>[2x]GSHMSI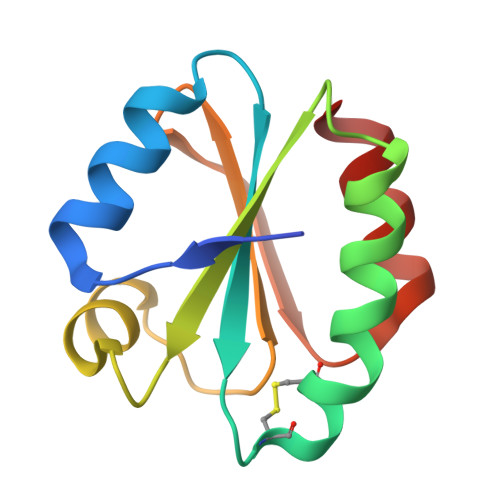HIKDSDDLKTRLAEAGDKLVVIDFMATWCGPCKMIGPKLDEMAGEMQDSIVVVKVDVDECEDIATEYNINSMPTFVFVKNGKKIEEFSGANVDKLRNTILKLK> DFVERQQWLAQPPQKEIPDLELPVGLVIALPTNSENCSTQAICVLRVRLLQTYDIESSQKCDIAYNFLIGGDGNVYVGRGWNKMGAHMNNINYDSQSLSFAYIGSFKTIQPSAKQLSVTRLLLERGVKLGKIAPSYRFTASSKLMPSVT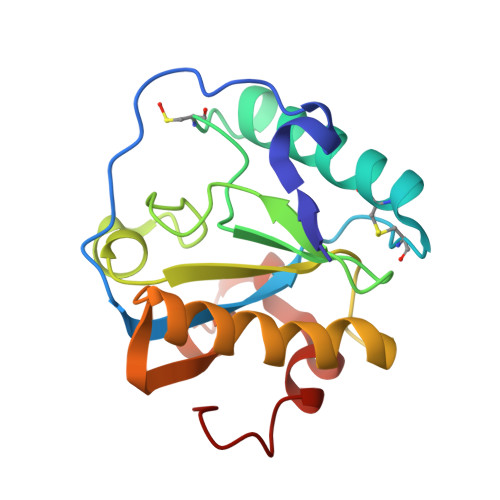DFKADALYASFANWTHWS>[2x]GHMDTPVLTPTEAAVLRELRLHRPQLPLDTLLFTDPNKDPDDVVTYTIAKQLQADGFLRLTDVVVTLGDADMRSQRAQLAKGVFDRLALPDVRVARGQDYPMTSTQAREHSKFLAEGAALR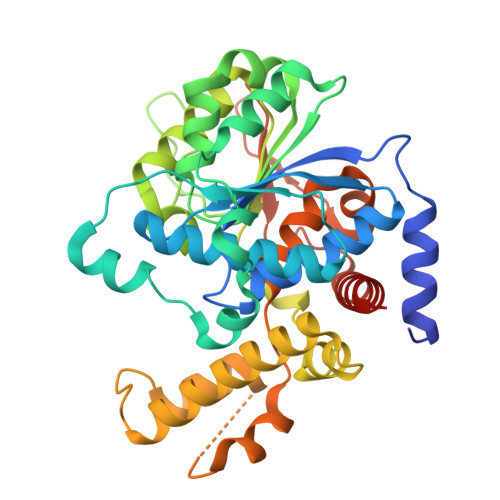AAPDAVHTDGVRAMCERLATSPHKLGMVVIAGMTDASALLAEAGDLVREKVASITIMGGIDPARDADGLVQPDTRAYNNATDIHAARALYRRAQQLGIPLRILTKEAAYKAAVPPAFYEGIARNGHPVGEYLRDVQKNALKGLWEGIQANLIPGLDTAWFFRTFVAAQPQDPVAADQQGALSFDAIWPQVTKLNLYDPLTLLAALPGTARLLFQPTPMHREGASPVEHVGHAEVVRPEKARLLLSALAKAALVQQDEGEHAR The centromere binding factor 3 (CBF3) complex binds the third centromere DNA element in organisms with point centromeres, such as S. cerevisiae. It is an essential complex for assembly of the kinetochore in these organisms, as it facilitates genetic centromere specification and allows association of all other kinetochore components. CBF3 comprises two homodimers, of Cep3 and Ndc10, and a Ctf13-Skp1 heterodimer. Cep3 provides sequence specificity through binuclear zinc-cluster (Zn2Cys6) domains homologous to those found in GAL4-like fungal transcription factors (Lechner, 1994, MacPherson et al., 2006).

In order to identify the binding site for Ndc10 on CBF3CCΔN we assembled a complex of CBF3CCΔN bound to a monomeric construct of Ndc10 comprising domains 1 and 2 (Ndc10 D1-2). Two-dimensional classification revealed high-resolution classes in which secondary structural elements could be identified, and these data generated a 4.2 Å map. Our map of the complex between CBF3CCΔN and Ndc10 D1-2 has excellent density for the core complex and lower resolution for Ndc10, suggesting flexibility between the two. Focused refinement of Ndc10 D1-2 yielded a second map with improved density for Ndc10. The atomic model of CBF3CCΔN fits readily into our composite map, and the remaining density accommodates the crystal structure of S. cerevisiae Ndc10 D1-2. Ndc10 binds to the F box of Ctf13 on the outside of the channel, and two unique structural elements of this atypical F box are responsible for the interaction. Specifically, within Ctf13, the long insertion between α2 and α3 (approximately amino acids 30–90), which is predicted to be helical and contains stretches of conservation particularly through residues 70–90, and a turn between β2 and β3 of the antiparallel β sheet, locate to density at the interface with Ndc10 D1-2. The interface on Ndc10 is mediated primarily by residues at its N terminus (before Gln 44) which are also predicted to be helical, with minor contributions from the C-terminal end of α3 (Val138) and a disordered loop between α1 and α2 (Pro65–Ser72). The C-terminal residues of Skp1 (Glu189–Arg194) are also located at the interface. Superposition of the crystal structure of DNA-bound Ndc10 D1-2 from the budding yeast Kluyveromyces lactis onto our model indicates that the DNA-binding site of Ndc10 is coplanar with, and approximately perpendicular to, the CBF3CCΔN channel.

>[2x]MGGSSHHHHHHSSGLVPRGSHMKLITASSSKEYLPDLLLFWQNYEYWITNIGLYKTKQRDLTRTPANLDTDTEECMFWMNYLQKDQSFQLMNFAMENLGALYFGSIGDISELYLRVEQYWDRRADKNHSVDGKYWDALIWSVFTMCIYYMPVEKLAEIFSVYPLHEYLGSNKRLNWEDGMQLVMCQNFARCSLFQLKQCDFMAHPDIRLVQAYLILATTTFPYDEPLLANSLLTQCIHTFKNFHVDDFRPLLNDDPVESIAKVTLGRIFYRLCGCDYLQSGPRKPIALHTEVSSLLQHAAYLQDLPNVDVYREENSTEVLYWKIISLDRDLDQYLNKSSKPPLKTLDAIRRELDIFQYKVDSLEEDFRSNNSRFQKFIALFQISTVSWKLFKMYLIYYDTADSLLKVIHYSKVIISLIVNNFHAKSEFFNRHPMVMQTITRVVSFISFYQIFVESAAVKQLLVDLTELTANLPTIFGSKLDKLVYLTERLSKLKLLWDKVQLLDSGDSFYHPVFKILQNDIKIIELKNDEMFSLIKGLGSLVPLNKLRQESLLEEEDENNTEPSDFRTIVEEFQSEYNISDILS;> MGVTSNVVLVSGEGERFTVDKKIAERSLLLKNYLNDMHDSNLQNNSDSESDSDSETNHKSKDNNNGDDDDEDDDEIVMPVPNVRSSVLQKVIEWAEHHRDSNFPDEDDDDSRKSAPVDSWDREFLKVDQEMLYEIILAANYLNIKPLLDAGCKVVAEMIRGRSPEEIRRTFNIVNDFTPEEEAAIRRENEWAEDRGS;> MGPSFNPVRFLELPIDIRKEVYFHLDGNFCGAHPYPIDILYKSNDVELPGKPSYKRSKRSKKLLRYMYPVFATYLNIFEYSPQLIEKWLEYAFWLRYDCLVLDCFKVNHLYDGTLIDALEWTYLDNELRLAYFNKASMLEVWYTFKEYKKWVIDSVAFDELDLLNVSNIQFNIDNLTPQLVDKCLSILEQKDLFATIGEVQFGQDEEVGEEKDVDVSGANSDENSSPSSTIKNKKRSASKRSHSDNGNVGATHNQLTSISVIRTIRSMESMKSLRKITVRGEKLYELLINFHGFRDNPGKTISYIVKRRINEIRLSRMNQISRTGLADFTRWDNLQKLVLSRVAYIDLNSIVFPKNFKSLTMKRVSKIKWWNIEENILKELKVDKRTFKSLYIKEDDSKFTKFFNLRHTRIKELDKSEINQITYLRCQAIVWLSFRTLNHIKLQNVSEVFNNIIVPRALFDSKRVEIYRCEKISQVLVIGSRSGSENLYFQGSKRRWKKNFIAVSAANRFKKISSSGAL;> MGRSSILFLLKLMKIMDVQQQQEAMSSEDRFQELVDSLKPRTAHQYKTYYTKYIQWCQLNQIIPTPEDNSVNSVPYKDLPISAELIHWFLLDTLITDDKPGEKREETEDLDEEEENSFKIATLKKIIGSLNFLSKLCKVHENPNANIDTKYLESVTKLHTHWIDSQKAITTNETNNTNTQVLCPPLLKVSLNLWNPETNHLSEKFFKTCSEKLRFLVDFQLRSYLNLSFEERSKIRFGSLKLGKRDRDAIIYHKVTHSAEKKDTPGHHQLLALLPQDCPFICPQTTLAAYLYLRFYGIPSVSKGDGFPNLNADENGSLLQDIPILRGKSLTTYPREETFSNYYTTVFRYCHLPYKRREYFNKCNLVYPTWDEDTFRTFFNEENHGNWLEQPEAFAFPDKIPFDFKKIMNFKSPYTSYSTNAKKDPFPPPKDLLVQIFPEIDEYKRHDYEGLSQNSRDFLDLMEVLRERFLSNLPWIYKFFPNHDIFQDPIFGNSDFQSYFNDKTIHSKGSPILSFDILPGFNKIYKNKTNFYSLLIERPSQLTFASSHNPDTHPWSHPQFEK>[2x]ACC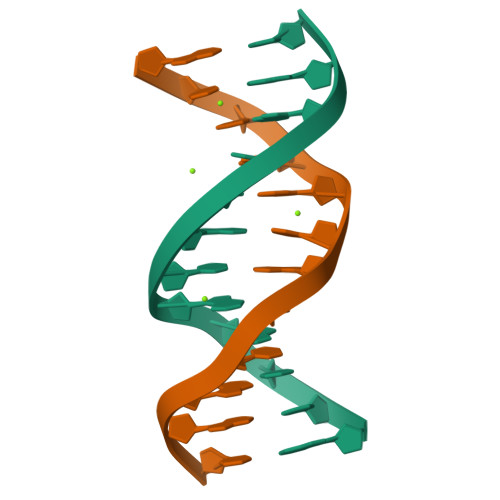GACGTCGGT> GPHMMVSDLKFAPSFQSFVDSSFFHELSRLKLDIFKLDSDEKALYTQLDLNQFTSNV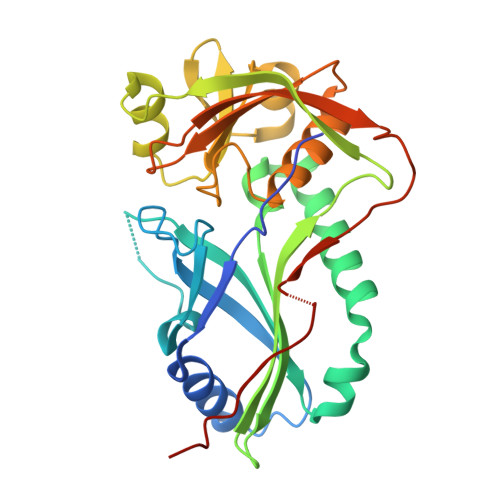LAISLRDDSFQKPDNDEHNIILKGYLLNFNTIELFKNCNKIQFIKEKGQELLQRGLENDLNEIISFYMISFADLKKYKFYYWICMPSFQSDGATYQIISSKVIASDSDISVSFIKQNVIIACVISGVIQKATPDNLKVCEKVVFKDFSHLKDIPSAVTKNILTVWSKLSPRETYTICFLRSDESSFEAEIIINNGNNPSLKVSGWEKNGLGKLAPKSIDLSSLMDP>AEAGITGTWYNQLGSTFIVTAGADGALTGTYESAVGNAESRYVLTGRYDSAPATDGSGTALGWTVAWKNNYRNAHSATTWS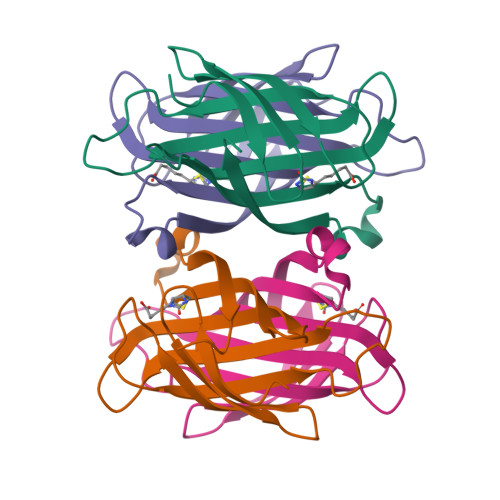GQYVGGAEARINTQWLLTSGTTEANAWKSTLVGHDTFTKVKPSAAS[4x]> GSHMRKQLFFTLARPCVAVGRRFISGDNKSIDSSAFISDDDALRGELASALDTEGHALPFDVHLQQPHSSGDGTAGDTSTIQLEKLSHPPARFDLLTNSFVYKWQTKAALARKVSGPMREWAAELKYRTGVHIELEPTYPERLSENAVKGSGSDDGDGTQWGAYETADDVDITVYLFGSERGIFNCHKLMEAAIQQDPVYVRLGIFRRLANSSEVEWLMLRRINRELRPPDIPPISLKLPGKWTLLYERYKEAAIRTLWEETGITVDASNVYPTGHLYQTVPQYYWRVPVRYFVAEVPSDIRVEGPQVVPLQYMRNWDARLLRQSPDPIDRAWAQLADPATGCAWMKASMIDQLQKPLRGDNYMAIRYTPPPYSNLQEVVGLGDGSITPSTGNGEDAS

The 5′ ends are processed by a pyrophosphohydrolase complex termed the PPsome, which is composed of the so-called mitochondrial edited mRNA stability factors 1–3 (MERS1–MERS3). MERS1 was shown to be the factor responsible for catalyzing the 5′ processing event while MERS2 and MERS3 activates its catalysis. Interestingly, the MERS1 Nudix motif (KWTLLYERYKEAAIRTLWEETGI) lacks one of the key metal ion coordinating acidic residues, which in MERS1 is a threonine instead of an acidic residue. The MERS1 structure reveals that it is comprised of two α−β domains.

Apo MERS1 crystals were grown and the structure was solved using the MERS1–GDP structure (after removing the GDP molecule) as a search model in molecular replacement (MR). A clear solution was obtained and the structure was refined to final Rwork/Rfree values of 18.8%/20.9% to 2.30 Å resolution. The apo MERS1 adopts a different crystal form with distinct packing compared to the MERS1–GDP structure and as a result we did not see the fortuitously bound helix in the apo structure. Comparison of the apo and GDP bound MERS1 structure revealed that the N-domain and most of the C-domain have the same structure; the two structures can be superimposed with a rmsd of 0.9 Å for 260 corresponding Cα atoms. There is, however, a notable difference between the two structures at the base of C-domain near the GDP binding pocket. Specifically, in the apo structure density was absent for the region encompassing residues 354–380. This region contains key residues involved in nucleotide binding, including Arg356, Tyr360, Arg364, and Tyr365. In fact, the RNA is deeply embedded in MERS1, raising the question of how it gains entry into this binding site. This appears to be explained by the apo MERS1 structure, which revealed that a key part of the RNA binding region is disordered in the apo state. The binding and stabilization of the single-stranded RNA may thus occur concomitant with the folding of MERS1 residues 354–380.> GPMVVNQKISGLASAMNAKIIGSGERSMVLAHGFGGDQSVWDKIIPVLSQSFKVLVFDWLFSGAIKDQTLYDPSKYNSLDVFSDDLIALMEELKFGPVVFVGHSMSGVIGCAASIKRPDLFTNLLLIAASPRYINSEDYKGGFE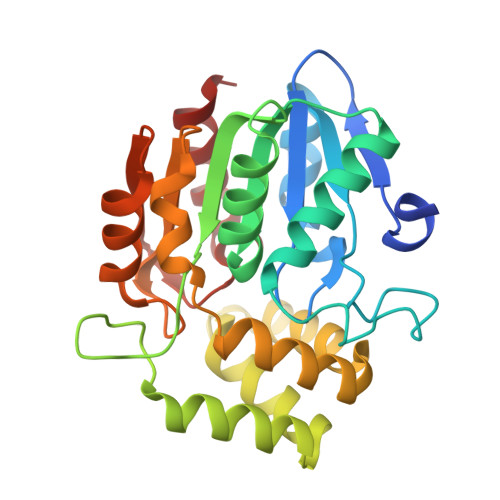SKDIDTIITSIGSNYEAWAVDFSSFVVDSRDSLSVQRFEKSLKKMKPETALALAKIVFGSDEREILGQVSVPCHVIQPGNDVVVPVSVAYFMQEKIKGKSTVEIIEDAIGHFPQMTSHLELLGVMRRLLEF> AGCGAAC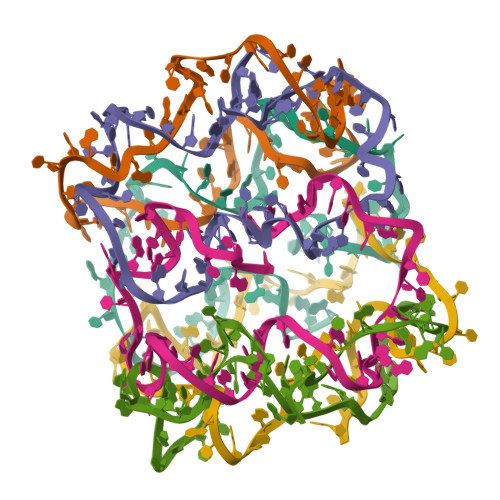GTGGATTTTGTCCGACATCGGCAAGCTCCCTTTTTCGACTATT;> CCGATGTCGGACTTTTACACGATCTTCGCCTGCTGGGTTTTGGGAGCTTG;> CGAAGATCGTGTTTTTCCACAGTTGATTGCCCTTCACTTTTCCCAGCAGG;> AATCAACTGTGGTTTTTCTCACTGGTGATTAGAATGCTTTTGTGAAGGGC;> TCACCAGTGAGATTTTTGTCGTACCAGGTGCATGGATTTTTGCATTCTAA;> CCTGGTACGACATTTTTCCACGTTCGCTAATAGTCGATTTTATCCATGCA> LKESPSGYLRSGEGDTGCGELVWVGEPLTLRTAETI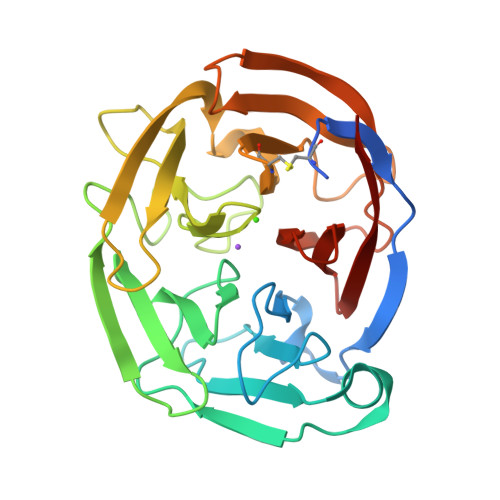TGKYGVWMRDPKPTYPYTQETTWRIDTVGTDVRQVFEYDLISQFMQGYPSKVHILPRPLESTGAVVYSGSLYFQGAESRTVIRYELNTEIVKAEKEIPGAGYHGQFPYSWGGYTDIDLAVDEAGLWVIYSTDEAKGAIVLSKLNPENLELEQTWETNIRKQSVANAFIICGTLYTVSSYTSADATVNFAYDTGTGISKTLTIPFKNRYKYSSMIDYNPLEKKLFAWDNLNMVTYDIKLSKM> MAHHHHHHSSGLEVLFQGPEPKKYAVTDDYQLSKQVLGLGVNGKVLECFHRRTGQKCALKLLYDSPKARQEVDHHWQASGGPHIVCILDVYENMHHGKRCLLIIMECMEGGELFSRIQERGDQAFTEREAAEIM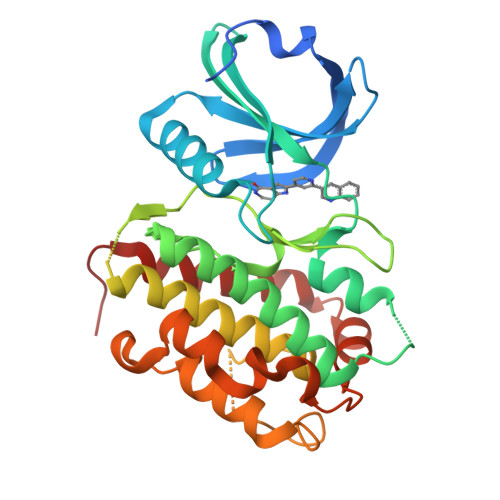RDIGTAIQFLHSHNIAHRDVKPENLLYTSKEKDAVLKLTDFGFAKETTQNALQTPCYTPYYVAPEVLGPEKYDKSCDMWSLGVIMYILLCGFPPFYSNTGQAISPGMKRRIRLGQYGFPNPEWSEVSEDAKQLIRLLLKTDPTERLTITQFMNHPWINQSMVVPQTPLHTARVLQEDKDHWDEVKEEMTSALATMRVDYDQV> MHNGWMSTAATAQEAQGLLLQLLDPATRADPYPIYDRIRRGGPLALPEANLAVFSSFSDCDDVLRHPSSCSDRTKSTIFQRQLAAETQPRPQGPASFLFLDPPDHTR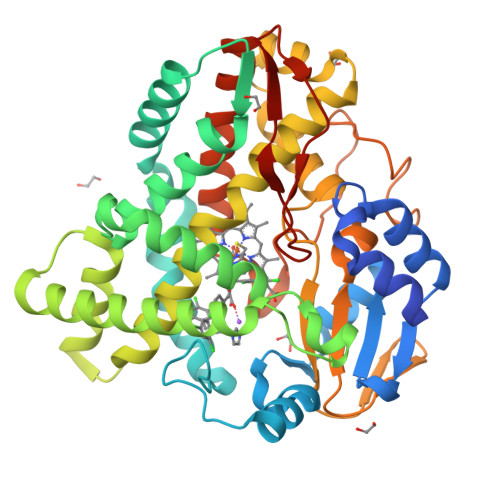LRGLVSKAFAPRVIKRLEPEITALVDQLLDAVDGPEFNLIDNLAYPLPVAVICRLLGVPIEDEPKFSRASALLAAALDPFLALTGETSDLFDEQMKAGMWLRDYLRALIDERRRTPGEDLMSGLVAVEESGDQLTEDEIIATCNLLLIAGHETTVNLIANAALAMLRTPGQWAALAADGSRASAVIEETMRYDPPVQLVSRYAGDDLTIGTHTVPKGDTMLLLLAAAHRDPTIVGAPDRFDPDRAQIRHLGFGKGAHFCLGAPLARLEATVALPALAARFPEARLSGEPEYKRNLTLRGMSTLSIAVHHHH>[2x]MNSPISPIETVPVKLKPGMDGPKVKQWPLTEEKIKALVEICTEMEKEGKISKIGPENPYNTPVFAIKKKDSTKWRKLVDFRELNKRTQDFWEVQLGIPHPAGLKKKKSVTVLDVGDAYFSVPLDEDFRKYTAFTIPSINNETPGIRYQYNVLPQGWKGSPAIFQSSMTKILEPFRKQNPDIVIYQYMDDLYVGSDLEIGQHRTKIEELRQHLLRWGLTTPDKKHQKEPPFLWMGYELHPDKWTVQPIVLPEKDSWTVNDIQKLVGKLNW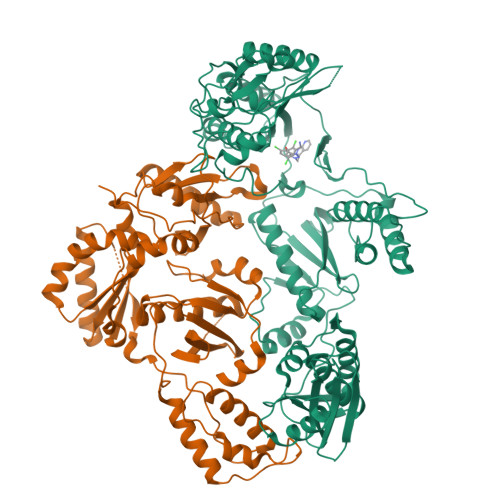ASQIYPGIKVRQLCKLLRGTKALTEVIPLTEEAELELAENREILKEPVHGVYYDPSKDLIAEIQKQGQGQWTYQIYQEPFKNLKTGKYARMRGAHTNDVKQLTEAVQKITTESIVIWGKTPKFKLPIQKETWETWWTEYWQATWIPEWEFVNTPPLVKLWYQLEKEPIVGAETFYVDGAANRETKLGKAGYVTNRGRQKVVTLTDTTNQKTELQAIYLALQDSGLEVNIVTDSQYALGIIQAQPDQSESELVNQIIEQLIKKEKVYLAWVPAHKGIGGNEQVDKLVSAGIRKVL> GPMDETGKELLLVLYDYQEKSPRELTCKKGDIL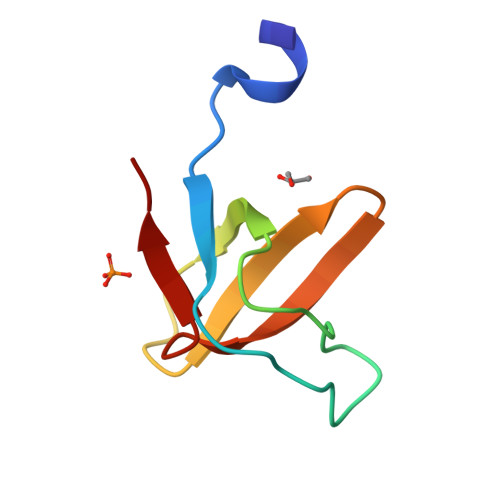TLLNSTNKDWWKVEWNDRQGFLPAAYLKKLD Thymidylate synthase (EC 2.1.1.45) catalyzes the dUMP methylation reaction, involving N5,10-methylenetetrahydrofolate (meTHF)-aided concerted transfer and reduction of the one-carbon group, its products being thymidylate and dihydrofolate (DHF). N4-hydroxy-2′-deoxycytidine 5′-monophosphate (N4-OH-dCMP) is a substrate analog, reported to inhibit the enzyme from bacterial, avian and mammalian sources, as well as from certain helminths. Inhibition was found to be competitive with respect to dUMP, and apparently mechanism-based, as it showed meTHF- and time-dependence; the dependence on time pointed to the slow-binding inhibition. Novel evidence is presented allowing further clarification of the mechanism of the slow-binding thymidylate synthase (TS) inhibition by N4-hydroxy-dCMP (N4-OH-dCMP).

Structural results provide further evidence that such incubation, also with the parasitic nematode T. spiralis enzyme, results in the inhibitor molecule being covalently bound at the active center via the pyrimidine C(6) and Cys189 sulfur, with the pyrimidine C(5) non-substituted by methyl, but acquiring an additional hydrogen atom. An asymmetric unit contains a single TspTS dimer. Residues 18–41 and 45–307 of chain A and 18–303 of chain B were modeled. Within each of the two active sites a clear electron density was present, identified as the N4-OH-dCMP molecule. However, no electron density was found that could be unequivocally identified as a folate derivative molecule. Both N4-OH-dCMP molecules were refined with high occupancy (0.95 and 0.93 in subunits A and B, respectively), with each N4-OH-dCMP pyrimidine ring conformation pointing to sp3 hybridizations of the C(5) and C(6) atoms, and the distance between pyrimidine C(6) and Sγ of Cys189 suggesting a covalent bond to be present between N4-OH-dCMP and each of TspTS subunits. The C-termini of the subunits A and B are in the open and closed conformations, respectively (the last four residues in subunit B were not modeled due to poor and ambiguous electron density). The C-terminus of subunit A is stabilized by crystal contacts with several residues from the neighboring TS dimer. Finally, minor conformational differences between mTS and TspTS could lead to faster DHF release from the latter.

>MKHHHHHHHMHAQMTETVHKLDTNSTSQDDYVNQEELNYLNQLKDIIDHGVRKNDRTGIGTLSTFGTQSRYCLRDDIFPLLTTKRVFWRGVVEELLWFISGSTNAKQLSEKNVNIWDGNSSREFLDSRGLYNYEEGDLGPVYGFQWRHFGCPYSSMTADYKGKGYDQLQQCIKMIREEPESRRIIMTAWNPCDLEKVALPPCHCFVQFYVADGELSCQMYQRSADMGLGVPFNIASYSLLTRMIAHITSLKPGFFIHTIGDAHVYLTHVDALKVQMERKPRPFPKLKILRNVENIDDFRAEDFELINYKPYPKISMPMAV[2x]ToxT is an AraC-family transcriptional activator of Vibrio cholerae virulence-gene expression, with a C-terminal DNA-binding domain and an N-terminal domain involved in dimerization and effector binding. ToxT directly activates the expression of the genes encoding the toxin-coregulated pilus (TCP), which is essential for colonization of the human intestine, and the cholera toxin (CT), the cause of the diarrheal disease that is characteristic of cholera. In V. cholerae, ToxT-dependent gene activation is inhibited by both bile and individual unsaturated fatty acids found in bile. Although oleic acid is likely to be the physiological effector of ToxT given its high concentration in bile, both PAM and oleic acid have been shown to reduce the expression of tcp and ctx in vivo and to reduce DNA binding by ToxT in vitro.

However, the structure determined by Lowden et al. contains a disordered region between residues Asp101 and Glu110 within the N-terminal domain. Interestingly, Asp101–Glu110 could be modeled in this structure, which included helix α1 and a loop region that connects this helix to the β9 sheet. In this region, helix α1 spans Ser87–Ile98 and contains a kink at Leu94. This is followed by a 310-helix spanning Leu99–Asp101 that continues into a shorter helix from Leu102 to Leu107 (α1′). Tyr108–Asp113 form a connecting loop between α1′ and β9. This region appears to be stabilized by residue Glu156, in helix α3, through a salt bridge with residue Arg105. Interestingly, the ToxT region between α1 and β9 (residues Asp101–Glu110) is folded over a loop that is located sequentially after it: the loop that connects helices α3 and α4, spanning residues Lys158–Ala170. Our structure suggests the possibility that Arg105 holds Glu156 in a position that somewhat attenuates ToxT activity. In addition, three chloride ions were modeled in the C-terminal region of ToxT, which were assigned based on the coordination distances (∼3.1–3.3 Å) to neighboring residues and water molecules. Overall, the new structure provides more complete, detailed and higher quality structural information for ToxT than the previously determined ToxT structure.

> MIGKKSFQTNVYRMSKFDTYIFNNLYINDYKMFWIDSGIAKLIDKNCLVSYEINSSSIILLKKNSIQRFSLTSLSDENINVSVITISDSFIRSLKSYILGDLMIRNLYSENKDLLLWNCEHNDIAVLSEVVNGFREINYSDEFLKVFFSGFFSKVEKKYNSIFITDDLDAMEKISCLVKSDITRNWRWADICGELRTNRMILKKELESRGVKFRELINSIRISYSISLMKTGEFKIKQIAYQSGFASVSYFSTVFKSTMNVAPSEYLFMLTGVAEK> MKLAL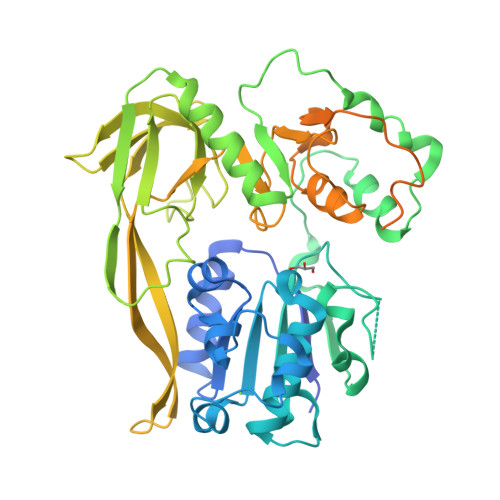NTEFKKAIDLATNSSKNLFITGKAGTGKSTFLKYLINELLFDAVVLAPTGVAAINIGGETIHSFFNFPINITPDKIPDLFIYDYEIYKYVNTIIIDEISMVRADLLDCIDLFLKRVKNPKLPFGGTKMIFIGDLYQLPPVLTNHQKKAFNMEYESPYFFSAKVFKEMDMEFIEFETIYRQSDKLFIDILNRIRNNTVTDEDIKIINSRVQDKIDNDDGYIYITTVNKKAEEINNQKLDKLKGKLYKLNGTLKGNFDENSLPTPKNLHLKIGAQVMLLNNAPDRMWVNGTIGTITNIFPDEMIIELALENGNIVEITPFKWDMIKFTYDKKEKKMLSETIGSYTQFPLKLAYAITVHKSQGKTFHKVIIDTSRHFFAPGQFYVALSRCTSLDGIILTKKITKNSIILDKKVVNFLTNFQYQLSEKKTPLEEKISILKRAIERNSPLEIVYLKTKDEKSKRVIIPKEVGEMVYSGKSFMGLKGFCTMRNDERVFRIDRILEIKEIND> MVSVINTVDTSHEDMIHDAQMDYYGTRLATCSSDRSVKIFDVRNGGQILIADLRGHEGPVWQVAWAHPMYGNILASCSYDRKVIIWREENGTWEKSHEHAGHDSSVNSVCWAPHDYGLILACGSSDGAISLLTYTGEGQWEVKKINNAHTIGCNAVSWAPAVVPGSLIDHPSGQKPNYIKRFASGGCDNLIKLWKEEEDGQWKEEQKLE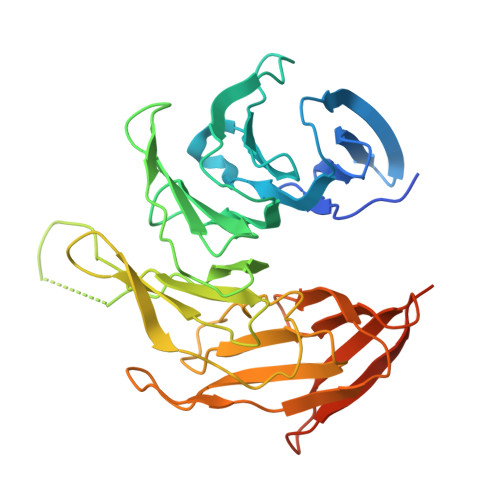AHSDWVRDVAWAPSIGLPTSTIASCSQDGRVFIWTCDDASSNTWSPKLLHKFNDVVWHVSWSITANILAVSGGDNKVTLWKESVDGQWVCISDVNKGQGSVSASVTEGQQNEQ> GSHMNTAEEDMEDDTSWRSEATFQFTVERFSRLSESVLSPPCFVRNLPWKIMVMPRFYPDRPHQKSVGFFLQCNAESDSTSWSCHAQAVLKIINYRDDEKSFSRRISHLFFHKENDWGFSNFMAWSEVTDPEKGFIDDDKVTFEVFVQADAPHGVAWD

Herpesvirus-associated ubiquitin-specific protease (HAUSP, also known as USP7), a deubiquitylating enzyme of the ubiquitin-specific processing protease family, specifically deubiquitylates both p53 and MDM2, hence playing an important yet enigmatic role in the p53–MDM2 pathway. Here we demonstrate that both p53 and MDM2 specifically recognize the N-terminal tumor necrosis factor–receptor associated factor (TRAF)–like domain of HAUSP in a mutually exclusive manner. The crystal structures of the HAUSP TRAF-like domain in complex with p53 and MDM2 peptides, determined at 2.3-Å and 1.7-Å resolutions, respectively, reveal that the MDM2 peptide recognizes the same surface groove in HAUSP as that recognized by p53 but mediates more extensive interactions. Structure-based sequence alignment of the three HAUSP-binding peptides revealed a conserved four-residue binding motif with the consensus sequence of (Ø/E)-G-(Ø/G)-S, where Ø denotes a non-polar residue.

We crystallized this domain (residues 53–206) and determined its structure at 1.65-Å resolution. As previously reported, the HAUSP TRAF-like domain adopts an eight-stranded anti-parallel β-sandwich structure, with strands β1, β5, β6, and β8 in one sheet and strands β2, β3, β4, and β7 in the other. The overall structure of the HAUSP TRAF-like domain closely resembles the TRAF-C domain of the TRAF family of proteins. In addition, the HAUSP TRAF-like domain contains a shallow surface groove in the middle of the β-sandwich, which corresponds to the region where the receptor peptides bind. The fact that most of the conserved peptide-binding residues in TRAFs are no longer present in the structure of the HAUSP TRAF-like domain indicates that the TRAF-like domain of HAUSP represents a new peptide-binding motif in the TRAF family.> SQPIFLNVLEAIEPGVVCAGHDNNQPDSFAALLSSLNELGERQLVHVVKWAKALPGFRNLHVDDQMAVIQYSWMGLMVFAMGWRSFTNVNSRMLYFAPDLVFNEYRMHKSRMYSQCVRMRHLSQEFGWLQITPQEFLCMKALLLFSIIPVDGLKNQKFFDELRMNYIKELDRI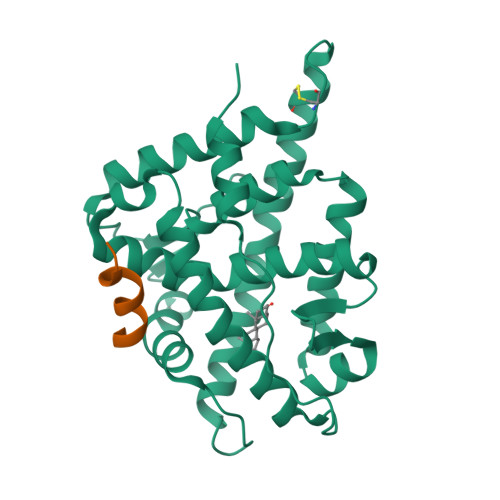IACKRKNPTSCSRRFYQLTKLLDSVQPIARELHQFTFDLLIKSHMVSVDFPEMMAEIISVQVPKILSGKVKPIYFHT;> HKKLLQLLTCSS The biosynthesis of neurotoxin aetokthonotoxin (AETX) that features a unique structure of pentabrominated biindole nitrile involves a first-of-its-kind nitrile synthase termed AetD, an enzyme that shares very low sequence identity to known structures and catalyzes an unprecedented mechanism. AetD adopts the heme oxygenase like fold and forms a hydrophobic cavity within a helical bundle to accommodate the indole moiety. A diiron cluster comprising two irons that serves as a catalytic center binds to the carboxyl O and the amino N of the substrate. Akak et al. conducted biochemical analyses and confirmed that Fe(II) is required for AetD activity and the nitrogen atom in the nitrile is sourced from the α-amino group of the substrate instead of exogenous nitrogen or the enzyme residue.

Notably, we demonstrate that the AetD-catalyzed reaction is independent of the bromination of the substrate and also solved crystal structures of AetD in complex with 5-Br-L-Trp and L-Trp. We also solved the crystal structure of AetD in complex with 2 and 3, which reveal that these compounds bind in the pocket as that was observed in AetD/1/Fe. In addition, the structures of these complex crystals without soaking with Fe ion were also solved. These complexes harbor the same metal ion coordination statuses as that was observed in the AetD/1 structure, which provide additional evidences to support the conclusions regarding the formation of the diiron cluster in AetD/Fe complex crystals. Notably, 2 lacks the S214-mediated interaction and 3 forms even fewer contacts to the enzyme in comparison with 1 and 2. This could be one factor accounting for the lower transformation efficacy of 3.

>[2x]AGAGAGAGAGMKAILQLILEKRQEFEKLPCFEFVRDETISPEERLILYPCIAAFALNFRDLNRYDYRDDNSSDYYQKIINIHTQEDAKHWEWFLNDLELLGFDKTMRFSEALRFVWSDDLLHTRRLCHNIAVLSHDLEPVMKMVVIEAMETAGLVIFHALAKPGESIAKATRRKYLYVADSHVEVETGHAVGTENIITILEQTQLSSEQEEKAKEIVNKVFQWSTNLIGEFERYVKAHRSEKAQPTAAY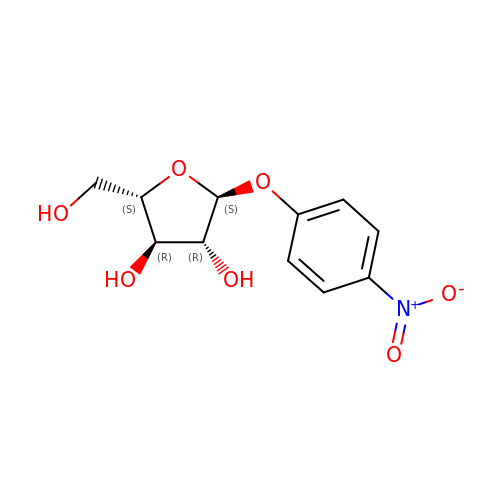4-nitrophenyl alpha-L-arabinofuranoside | C11 H13 N O7 | DUYYBTBDYZXISX-UKKRHICBSA-N3-bromanyl-5-(2-ethylimidazo[1,2-a]pyridin-3-yl)carbonyl-2-oxidanyl-benzenecarbonitrile | C17 H12 Br N3 O2 | 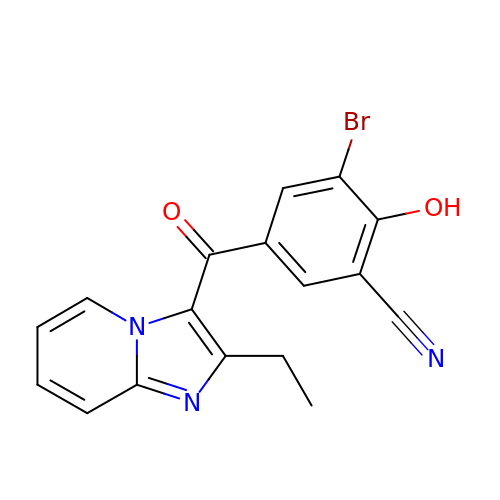RQGCKMOCOOAGEG-UHFFFAOYSA-N> GLIRQQIEYKTLILNCVNPDNENSPEIPVKVLNCDTITQVKEKILDAVYKNVPYSQRPRAVDMDLEWRQGRIARVVLQDEDITTKIEGDWKRLNTLMHYQVSDRSVVALVPK;> MHHHHHHSSGRENLYFQGRAPQPVVARCKLVLVGDVQCGKTAMLQVLAKDCYPETYVPTVFENYTACLETEEQRVELSLWDTSGSPYYDNVRPLCYSDSDAVLLCFDISRPETVDSALKKWRTEILDYCPSTRVLLIGCKTDLRTDLSTLMELSHQKQAPISYEQGCAIAKQLGAEIYLEGSAF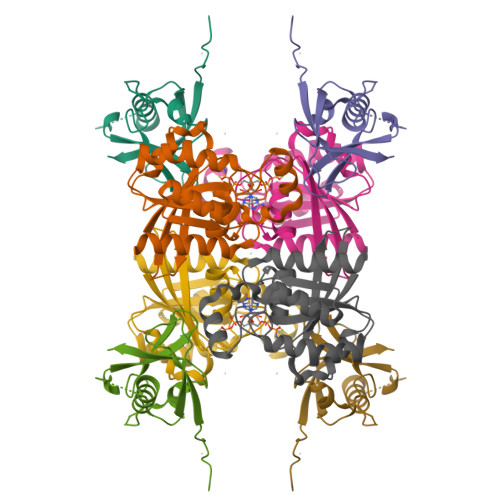TSEKSIHSIFRTASMLCLNKPSPLPQKSPV SAP05 is an effector from a plant pathogenic phytoplasma that mediates the degradation of host transcription factors, including SPL and GATA family proteins, by hijacking the 26 S plant ubiquitin receptor RPN10 independently of substrate ubiquitination. Specifically, SAP05 folds into a tight globular structure consisting of a parallel five-stranded β-sheet (β1-β5). Although SAP05 carries a single domain, it utilizes two opposing surfaces (hereafter referred to as Lobe1 and Lobe2) to interact simultaneously with TFs and AtRPN10, forming a dumbbell-shaped structure, in which TFs and AtRPN10 have no direct surface contacts. In summary, SAP05 bridges the TFs mainly through electrostatic interactions with a hydrophobic core, whereas the SAP05-AtRPN10 interface comprises predominantly extensive hydrophobic contacts.

In addition to SPL5, SAP05 can also target plant SPL13, another member of the SPL family that plays an important role in the juvenile-to-adult vegetative transition and the vegetative-to-reproductive transition. By X-ray crystallography, we also obtained the complex structure of SAP05 with SPL13, structural analysis indicated that it shares a conserved interaction pattern observed in the SAP05-SPL5 structure, highlighting the evolutionary conservation of SPL family recognition by SAP05.

>[2x]GAPHEERVGDMRIVNITFSDINSIKNFQPFSQYFDFTLTGPRYNGNIAQFAMIWKIKNPPHNLLGVFFDNNTRDDEDDKYTLEELKQMGNGAKNMYIFWQYEQK;>GMPICLVDGCDSDFSNCREYHKRHKVCDVHSKTPVVTINGHKQRFCQQCSRFHALEEFDEGKRSCR[2x]>[2x]SECKPGATFENRTVDCGGVTIGTSCPNDSDKQKPLIILKNATVKNLRISASGGADGIHCDSGNCTIENVIWEDICEDAATNNGKTMTIVGGIAHNAKDGYGGKPD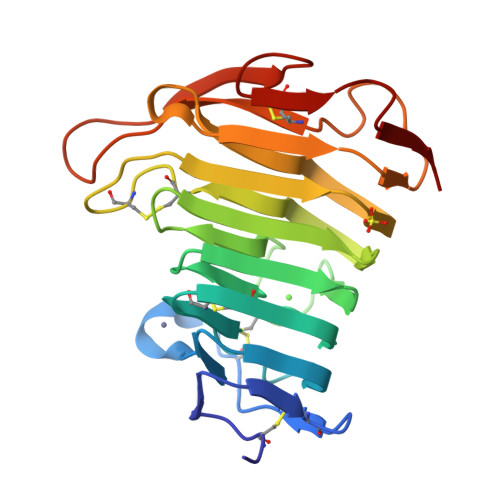KVLQHNSKNSTTVVKGNFTLTGEHGKLWRSCGDCSNNGGPRFLTVTSATVNGTIDSIAGVNRNYGDVATISGLKIKNYKEGKPPVCEEFKGVVKGQGSTEKYGEKWDTTNCKVSRSGVSKL> GFKVFGAPNVVEDEIDQYLSKQDGKIYRSRDPQLCRHGPLGKCVHCVPLEPFDEDYLNHLEPPVKHMSFHAYIRKLTGGADKGKFVALENISCKIKSGCEGHLPWPNGICTKCQPSAITLNRQKYRHVDNIMFENHTVADRFLDFWRKTGNQHFGYLYGRYTEHKDIPLGIRAEVAAIYEPPQIGTQNSLELLEDPKAEVVDEIAAKLGLRKVGWIFTDLVSEDTRKGTVRYSRNKDTYFLSSEECITAGDFQNKHPNMCRLSPDGHFGSKFVTAVATGGPDNQVHFEGYQVSNQCMALVRDECLLPCKDAPELGYAKESSSEQYVPDVFYKDVDKFGNEITQLARP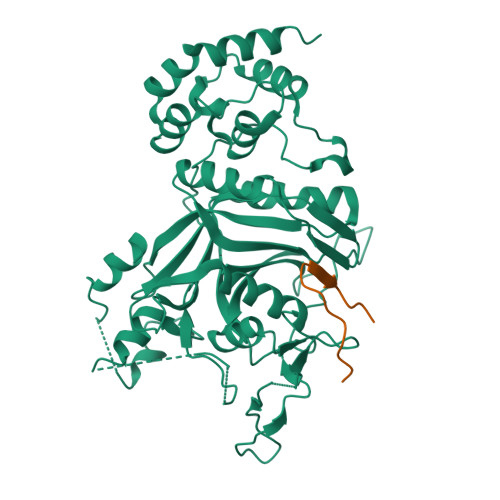LPVEYLIIDITTTFPKDPVYTFSISQNPFPIENRDVLGETQDFHSLATYLSQNTSSVFLDTISDFHLLLFLVTNEVMPLQDSISLLLEAVRTRNEELAQTWKRSEQWATIEQLCSTVG;> IPNYEFKLGKITFIRN> MEEKVESTTTPDGPCVVSVQETEKWMEEAMRMAKEALENIEVPVGCLMVYNNEVVGKGRNEVNQTKNATRHAEMVAIDQVLDWCHQHGQSPSTVFEHTVLYVTVEPCIMCAAALRLMKIPLVVYGCQNE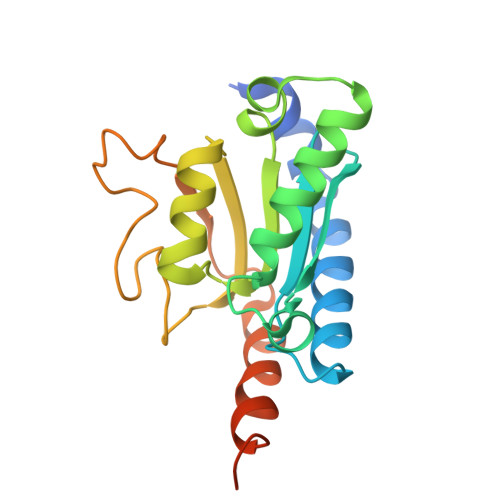RFGGCGSVLNIASADLPNTGRPFQCIPGYRAEEAVELLKTFYKQENPNAPKSKVRKKDCQKS> MEEKTVQVQKGLPSIDSLHYLSENSKKEFKEELSKAGQESQKVKEILAKAQQADKQAQELAKMKIPEKIPMKPLHGPLYGGYFRTWHDKTSDPTEKDKVNSMGELPKEVDLAFIFHDWTKDYSLFWKELATKHVPKLNKQGTRVIRTIPWRFLAGGDNSGIAEDTSKYPNTPEGNKALAKAIVDEYVYKYNLDGLDVAVLHDSIPKVDKKEDTAGVERSIQVFEEIGKLIGPKGVDKSRLFIMDSTYMADKNPLIERGAPYINLLLVQVYGSQGEKGGWEPVSNRPEKTMEERWQGYSKYIRPEQYMIGFSFYEENAQEGNLWYDINSRKDEDKANGINTDITGTRAERYARWQPKTGGVKGGIFSYAIDRDGVAHQPKKYAKQKEFKDATDNIFHSDYSVSKALKTVMLKDKSYDLIDEKDFPDKALREAVMAQVGTRKGDLERFNGTLRLDNPAIQSLEGLNKFKKLAQLDLIGLSRITKLDRSVLPANMKPGKDTLETVLETYKKDNKEEPATIPPVSLKVSGLTGLKELDLSGFDRETLAGLDAATLTSLEKVDISGNKLDLAPGTENRQIFDTMLSTISNHVGSNEQTVKFDKQKPTGHYPDTYGKTSLRLPVANEKVDLQSQLLFGTVTNQGTLINSEADYKAYQNHKIAGRSFVDSNYHYNNFKVSYENYTVKVTDSTLGTTTDKTLATDKEETYKVDFFSPADKTKAVHTAKVIVGDEKTMMVNLAEGATVIGGSADPVNARKVFDGQLGSETDNISLGWDSKQSIIFKLKEDGLIKHWRFFNDSARNPETTNKPIQEASLQIFNIKDYNLDNLLENPNKFDDEKYWITVDTYSAQGERATAFSNTLNNITSKYWRVVFDTKGDRYSSPVVPELQILGYPLPNADTIMKTVTTAKELSQQKDKFSQKMLDELKIKEMALETSLNSKIFDVTAINANAGVLKDCIEKRQLLKKLGSGKILHNQNVNSWGPITVTPTTDGGETRFDGQIIVQMENDPVVAKAAANLAGKHAESSVVVQLDSDGNYRVVYGDPSKLDGKLRWQLVGHGRDHSETNNTRLSGYSADELAVKLAKFQQSFNQAENINNKPDHISIVGCSLVSDDKQKGFGHQFINAMDANGLRVDVSVRSSELAVDEAGRKHTKDANGDWVQKAENNKVSLSWDA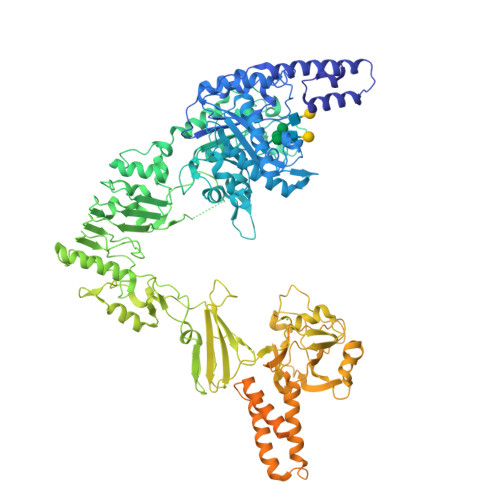QLEGGSGGSGNSGHHHHHHHHHH Our work utilizes biotin–streptavidin (Sav) technology to develop artificial metalloproteins (ArMs) that mimic the active sites of natural copper metalloenzymes. Our group develops artificial metalloproteins (ArMs) using biotin–streptavidin (Sav) technology to mimic natural metalloenzyme active sites to characterize otherwise elusive intermediates and study the effects of the secondary coordination sphere on metal ion(s) reactivity. This approach leverages the strong binding affinity between biotinylated metal complexes and the Sav host to confine synthetic metal cofactors within a protein scaffold. By engineering ArMs with aromatic residues within their secondary coordination spheres, we systematically investigate the influence of these residues on Cu reactivity and oxidant activation. Our results demonstrate how the inclusion of aromatic residues within the secondary coordination sphere influences the structure and reactivity of copper ArMs.

Based on the structures determined by XRD and the MS results, we sought to test whether the incorporation of a tyrosine residue at another location would lead to increase levels of non-specific protein oxidation and whether the oxidation of tyrosines in the secondary coordination sphere was influenced by their location relative to the Cu cofactor. We therefore incorporated our [CuII-biot-et-dpa] cofactor into a new variant in which K121 was substituted for a tyrosine, producing [CuII-biot-et-dpa⊂2XM-S112A-K121Y-Sav], where Y121 sits 6.7 Å from the copper center as determined by XRD (Fig. S23 and Table S2†). We note that despite being nearly equidistant to the Cu center as in 1, the interplay between tyrosine incorporation and N49 coordination is not observed in 3. This difference is likely because Y121 in 3 is unable to achieve the steric influence exerted by the positioning of Y112 in 1. However, comparison of the structures of 1 and 3 reveals differences in their primary coordination spheres, in which the amide residue at N49 no longer coordinates the Cu center in 3. Upon reacting with peroxide, whole-protein HR-ESI-Q-TOF MS of 3 showed oxidation levels that fell between those observed for 1 and 2. While peaks corresponding to singly and doubly oxidized species increased in relative abundance compared to those same features in 2, the base peak at 16 443.2 m/z still corresponds to the unoxidized protein, indicating that it remained the dominant species in solution. The surprising result that 3, with a tyrosine at 121, shows less modification of DF31 than 2 suggests that oxidation depends on the orientation and position of the Cu cofactor. We point out that while the oxidation of DF31 is limited in 3, the non-specific oxidation of other residues in 3 is enhanced relative to that in 2, an observation that is not yet completely understood.

> MASMTGGQQMGRDEAGITGTWYNQLGSTFIVTAGADGALTGTYESAVGNAESRYVLTGRYDSAPATDGSGTALGWTVAWKNNYRNAHSATTWSGQYVGGAQARINTQWLLTAGTTEANAWYSTLVGHDTFTKVKPSAASIDAAKKAGVNNGNPLDAVQQ>[2x]DSFWEVGNYKRTVKRIDDGHRLCGDLMNCLHERARIEKAYAQQLTEWARRWRQLVEKGPQYGTVEKAWIAVMSEAERVSELHLEVKASLMNEDFEKIKNWQKEAFHKQMMGGFKETKEAEDGFRKAQKPWAKKLKEVEAAKKAHHTACKEE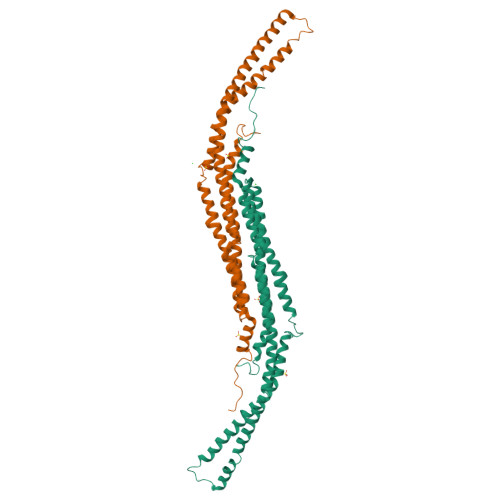KLAISREANSKADPSLNPEQLKKLQDKIEKCKQDVLKTKDKYEKSLKELDQTTPQYMENMEQVFEQCQQFEEKRLRFFREVLLEVQKHLDLSNVASYKTIYRELEQSIKAADAVEDLRWFRANHGPGMAMNWPQFE>[2x]AHPLENAWTFWFDNPQGKSRQVAWGSTIHPIHTFSTVEDFWGLYNNIHNPSKLNVGADFHCFKNKIEPKWEDPICANGGKWTISCGRGKSDTFWLHTLLAMIGEQFDFGDEICGAVVS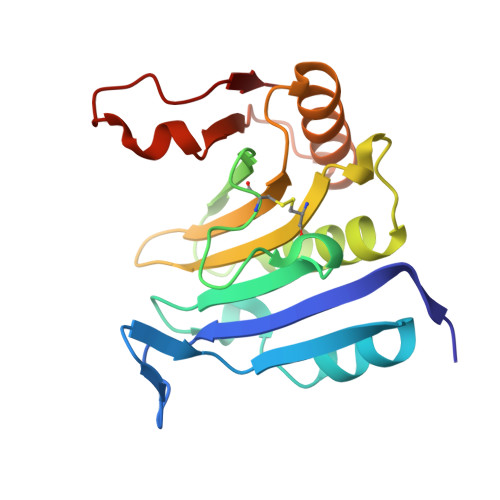VRQKQERVAIWTKNAANEAAQISIGKQWKEFLDYKDSIGFIVHEDAKRSDKGPKNRYTV>[3x]MGSSHHHHHHSQDPMNQPKNIFDEIYQETEKTYRLNNIFNKLTDVEVHSYQEYSDDSKFYPSILYKDIAKTGNYTKIAID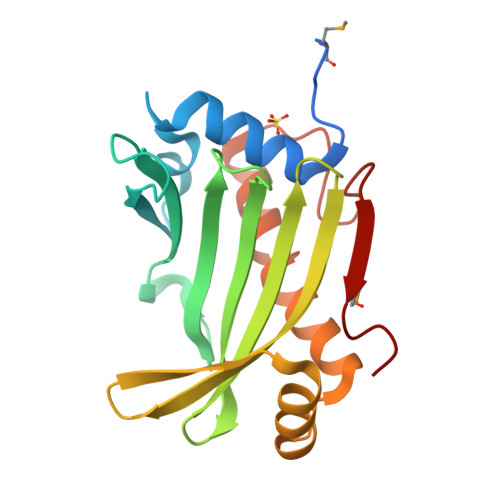FSFLNKNNNILIYFEKEIGPNVRVRIWNKYTRQDRTLTKSVKIALEKGDSDKYIEDETQVRAYLKKYGITAKDLDAHYEKIVNQKVLKDWCSIYKSKYSPKDYGQVTVKMQWEKW> MLRRSALARRYPFTKRGPRERKSWKHHVLTEPPKPVEWRDPKVWTKDLSQMKSFDAPQWDLWLNRSRSQDMDEALQPFMDMPQSLKDRRYDIPWWANPFGAWYLQNVLSVELMKLPGRTNAEKIAIYRGRKRPATWDKS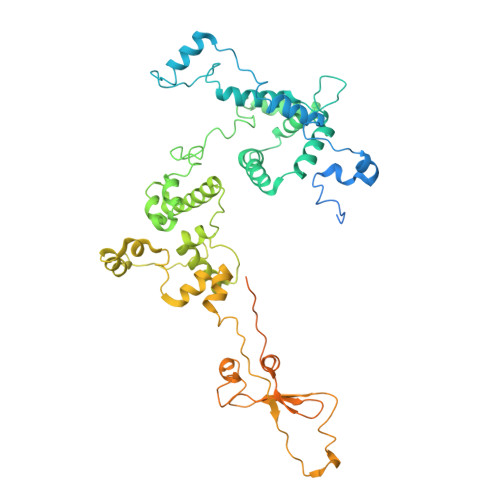KEGLMDDEVLLKQIVKERWRTLEFGDRDAGYPCTFSDYIQFLNEWFKSLDEEGLQRLREHFDRKIRPLLAVMTHVDLMWLEALTQNSVQNKEQLERRIGFQTSLGTPEFFDMSKRLRYEINEDYKVRDELGPELFALWSKAPERWPPERLAKMYGLDFTLVRKILVWHHFKACYDACVEPDWTLPKRLFALEWIRDVRARKQGLFYGKLRFAEQKITFYSDKFLFRDLVNRREASYANVWEMDDPYRFLQTEQDYEDYWGDNYDVYRRMFPEMIGKSGEPVQQYSQMPVWAGPHRDHANKSEHNWMFAEIGVNVGHEPLKKLELDPTNEKRRRFVIRQPDGSLRSAKMSEMRAWYWKEEWADFRFWAPHMEWGVENTPSMEQYQEHVPDTPDADYRKQRRIQSRPVKWFYESHYSRSGSFAGFQPLRFMQRRTQREVRWPDVINAAVQIEKSKPSSYVFKAIPEI>[2x]SGSGSTAEPDLKTALKAVIPAKRE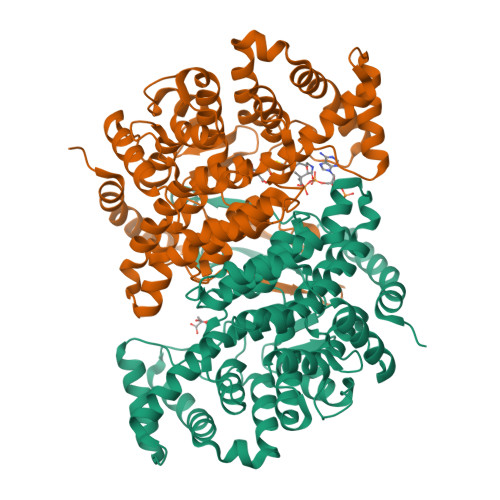LFKQVKERSDEVIGEVKVANVIGGMRGLKSMLWEGSVLDPEEGIRFHGKTIKDCQKELPKGTSGTEMLPEAMFWLLLTGQVPSTNQVRAFSRELAEQSHLPQHILDLIKSFPRSMHPMTQLSIAVAALNTESKFAKAYEKGLSKADYWEPTFDDSISLLAKIPRVAALVFRPDEVDQVGTQALDASQDWSYNFAELLGKGGKENQDFHDLLRLYLALHGDHEGGNVSAHATHLVGSALSDPFLSYSAGLLGLAGPLHGLAAQEVLRWILAMQDKIGTKFTDDDVRNYLWDTLKSGRVVPGYGHGVLRKPDPRFQALMDFAATRPDVLANPVFQLVKKNSEIAPAVLTEHGKTKNPHPNVDAASGVLFYHYGFQQPLYYTVTFGVSRALGPLVQLIWDRALGLPIERPKSINLLGLKK6-{[(3R,4R)-4-(2-{[2-(3-fluorophenyl)ethyl]amino}ethoxy)pyrrolidin-3-yl]methyl}-4-methylpyridin-2-amine | C21 H29 F 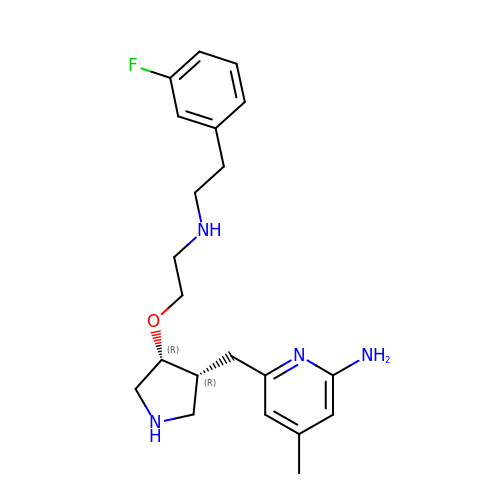N4 O | NESZTSPBRDBHCW-XLIONFOSSA-N DsbA from E. coli K−12 (EcDsbA) was the first and is probably the best-characterised DSB enzyme to date. This 21 kDa periplasmic protein is a dithiol oxidase that catalyses disulphide bond formation between consecutive cysteines of unfolded polypeptides as they are translocated to the periplasm. EcDsbA consists of a canonical TRX domain, a hallmark of proteins involved in redox homeostasis, with an inserted helical domain. The TRX domain harbours the conserved active site CXXC (C30-P31-H32-C33 in EcDsbA) that is featured in many proteins of the TRX superfamily. The acidity of this groove originates from a cluster of negatively charged residues (E24, E37, E38, D44, E85, D86 and E94) that map along a buried channel in the interface between the TRX and helical domains of EcDsbA.

DsbA K58A and double-mutant E24A/K58A were crystalised in space group C2, with two molecules per asymmetric unit. In comparison, overlay of chain A of wildtype DsbA and chain A of the E24A/K58A mutant showed the smallest difference, with an RMSD of 0.34 Å over 174 Cα atoms. The crystal structures of the three mutants containing the K58A mutation showed that the shorter alanine side chain at position 58 significantly expanded the size of the entrance to the buried channel. In all three crystal structures, a glycerol molecule, used for cryoprotection, was modelled into the electron density. The binding of glycerol displaced w2 in all three structures and hindered precise analysis of the water network in these mutants. When E37 was present in the protein structures, water w3 was observed to form a hydrogen bond with E37 in both K58A and E24A/K58A structures. However, the double-mutant E24A/K58A yielded a rate constant of 1.47 ± 0.06 × 106 M−1 s −1, 35% slower than that of wildtype EcDsbA. Mutation of two or more of the E24, E37 and K58 further increased the “disordered” solvent content, reducing the structured hydrogen bond network between the charged residues and the w1–w4 water molecules. Indeed, both E24A/K58A and E24A/E37A/K58A mutants displayed significantly lower thiol oxidase activity compared to the wildtype protein (although the more reducing redox potential of the latter would also affect its oxidase activity). While native DsbA rapidly oxidised the substrate peptide (in less than 10 s), in the case of the DsbA double E24A/K58A and triple E24A/E37A/K58A mutants, oxidised DsbA was present in the reaction for over 10 and 20 s, respectively.

>AQYEDGKQYTTLEKPVAGAPQVLAFFSFFCPHCYQFEEVLHISDNVKKKLPEGVKMTAYHVNFMGGDLGKDLTQAWAVAMALGVEDKVTVPLFEGVQKTQTIRSASDIRDVFINAGIKGEEYDAAWNSFVVKSLVAQQEKAAADVQLRGVPAMFVNGKYQLNPQGMDTSNMDVFVQQYADTVKYLSEKK[2x]> MSRSKRDNNFYSVEIGDSTFTVLKR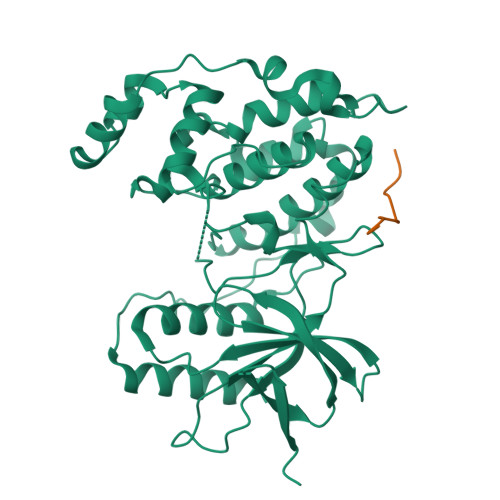YQNLKPIGSGAQGIVCAAYDAILERNVAIKKLSRPFQNQTHAKRAYRELVLMKVVNHKNIIGLLNVFTPQKSLEEFQDVYIVMELMDANLSQVIQMELDHERMSYLLYQMLVGIKHLHSAGIIHRDLKPSNIVVKSDATLKILDFGLARTAGTSFMMTPYVVTRYYRAPEVILGMGYKENVDIWSVGVIMGEMIKGGVLFPGTDHIDQWNKVIEQLGTPSPEFMKKLQPTVRTYVENRPKYAGYSFEKLFPDVLFPADSEHNKLKASQARDLLSKMLVIDASKRISVDEALQHPYINVWYDPSEAEAPPPKIPDKQLDEREHTIEEWKELIYKEVMDLEHHHHHH;> RPKRPTTLNLF The helicase domain of nonstructural protein 3 (NS3H) unwinds the double-stranded RNA replication intermediate in an ATP-dependent manner during the flavivirus life cycle. In this study, we focus on NS3H, which is a monomeric enzyme belonging to the DEAD/H box subfamily within the helicase superfamily 2 (SF2) and consists of three subdomains. The NTPase active site is located in a cleft between the subdomains 1 and 2 and involves motifs I (Walker A), II (Walker B), and VI. Here, we biochemically characterized NS3H from TBEV and obtained structures of key intermediates along the ATPase cycle (nucleotide-free, apo; ADP-; adenylyl-imidodiphosphate, AMPPNP-; and hydrolysis product, ADP–Pi-bound NS3H).

The apoNS3H protein crystallizes in space group P41212 at 1.83 Å. The refined model of apoNS3H (residues 173–621) is complete except for an N-terminal 10X-histidine tag region derived from the pET-19b vector together with a short flexible linker region between protease and helicase domains of NS3 (residues E173–Q181) and two nonconserved disordered loop regions (residues P251–G259 and T502–P506). Nonprotein positive 2Fo–Fc electron density was attributed to water molecules. NS3H has a clover-shaped architecture divided into three domains containing seven conserved motifs of SF2 helicase family. Domain 1 (residues W188–E329) consists of six β-strands surrounded by four α-helices, whereas domain 2 (residues P330–G486) consists of three α-helices and six β-strands with one antiparallel β hairpin passing close to domain 3. Domain 3 (residues L487–R621) consists of four α-helices and one β-hairpin. The empty NTPase site is filled with solvent molecules, and the P-loop adopts a “relaxed” conformation as found in ZIKV structure, whereas DENV helicase exhibits yet more open conformation. The resulting 3D protein structure shows overall similarity with already published helicase structures of other flaviviruses.

> MGHHHHHHHHHHSSGHIDDDDKHMEKSRPNLPQAVVGTGWTSKGQITVLDMHPGSGKTHRVLPELIRQCIDRRLRTLVLAPTRVVLKEMERALNGKRVRFHSPAVSDQQAGGAIVDVMCHATYVNRRLLPQGRQNWEVAIMDEAHWTDPHSIAARGHLYTLAKENKCALVLMTATPPGKSEPFPESNGAITSEERQIPDGEWRDGFDWITEYEGRTAWFVPSIAKGGAIARTLRQKGKSVICLNSKTFEKDYSRVRDEKPDFVVTTDISEMGANLDVSRVIDGRTNIKPEEVDGKVELTGTRRVTTASAAQRRGRVGRQDGRTDEYIYSGQCDDDDSGLVQWKEAQILLDNITTLRGPVATFYGPEQDKMPEVAGHFRLTEEKRKHFRHLLTHCDFTPWLAWHVAANVSSVTDRSWTWEGPEANAVDEASGDLVTFRSPNGAERTLRPVWKDARMFKEGRDIKEFVAYASGRR> SLAKSAANKLDWAKVISSLRITGSTATQLSSFKKRNDEARRQLLELQSQPTEVDFSHYRSVLKNTSVIDKIESYVKQYKPVKIDASKQLQVIESFEKHAMTNAKETESLVSKELKDLQSTLDNIQSARPFDELTVDDLTKIKPEIDAKVEEMVKKGKWDVPGYKDRFGNLNVM;> MPQLVPFYFMNQLTYGFLLMITLLILFSQFFLPMILRLYVSRLFISKL;> MLKRFPTPILKVYWPFFVAGAAVYYGMSKAADLSSNT;>MQLVLAAKYIGAGISTIGLLGAGIGIAIVFAALINGVSRNPSIKDTVFPMAILGFALSEATGLFCLMVSFLLLFGV[10x];> VSTLIPPKVVSSKNIGSAPNAKRIANVVHFYKSLPQGPAPAIKANTRLARYKAKYFDGDNASGKPLWHFALGIIAFGYSMEYYFHLRHHKGAEEH;> SPLDQFEIRTLFGLQSSFIDLSCLNLTTFSLYTIIVLLVITSLYTLTNNNNKIIGSRWLISQEAIY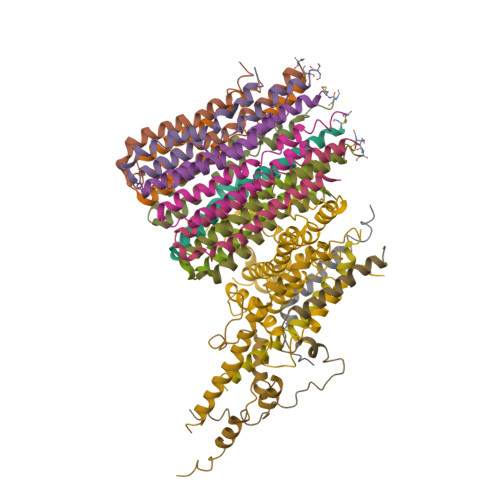DTIMNMTKGQIGGKNWGLYFPMIFTLFMFIFIANLISMIPYSFALSAHLVFIISLSIVIWLGNTILGLYKHGWVFFSLFVPAGTPLPLVPLLVIIETLSYFARAISLGLRLGSNILAGHLLMVILAGLTFNFMLINLFTLVFGFVPLAMILAIMMLEFAIGIIQGYVWAILTASYLKDAVYLH;> MSSTPEKQTDPKAKANSIINAIPGNNILTKTGVLGTSAAAVIYAISNELYVINDESILLLTFLGFTGLVAKYLAPAYKDFADARMKKVSDVLNASRNKHVEAVKDRIDSVSQLQNVAETTKVLFDVSKETVELESEAFELKQKVELAHEAKAVLDSWVRYEASLRQLEQRQLAKSVISRVQSELGNPKFQEKVLQQSISEIEQLLSKLK>[4x]ADDELYRQSLEIISRYLREQATGAKDTKPMGRSGATSRKALETLRRVGDGVQRNHETAFQGMLRKLDIKNEDDVKSLSRVMIHVFSDGVTNWGRIVTLISFGAFVAKHLKTINQESCIEP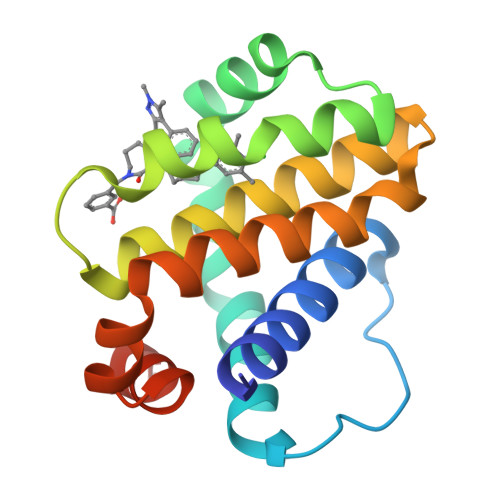LAESITDVLVRTKRDWLVKQRGWDGFVEFFHVEDLEGG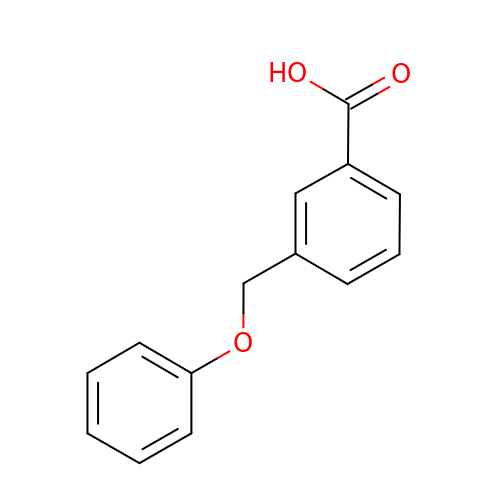3-(phenoxymethyl)benzoic acid | C14 H12 O3 | URLYREZIPSJJQU-UHFFFAOYSA-N>[6x]MKNGRLAGKRVLLTNADAYMGEATVQVFEEEG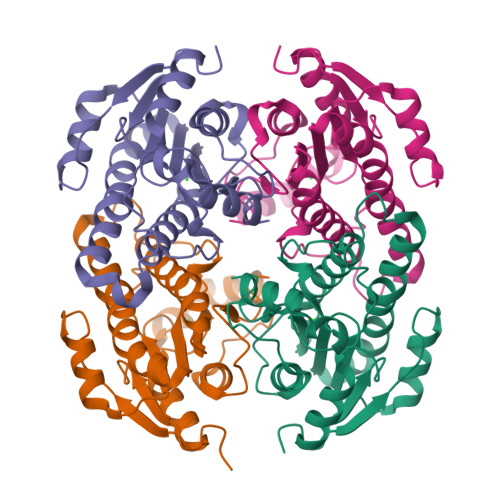AEVIADHTDLTKVGAAEEVVERAGHIDVLVANFAVDAHWGVTVLETDEELWQTAYETIVHPLHRICRAVLPQFYERNKGKIVVYGSAAAMRYTEGALAYSTARFAQRGYVTALGPEAARHNVNVNFIAQHWTQNKEYFWPERIATDEFKEDMARRVPLGRLATAREHALLALFLASDESDFIVGKSIEFDGGWAT>[3x]QDSTSDLIPAPPLSKVPLQQNFQDNQFQGKWYVVGLAGNAILREDKDPQKMYATIYEL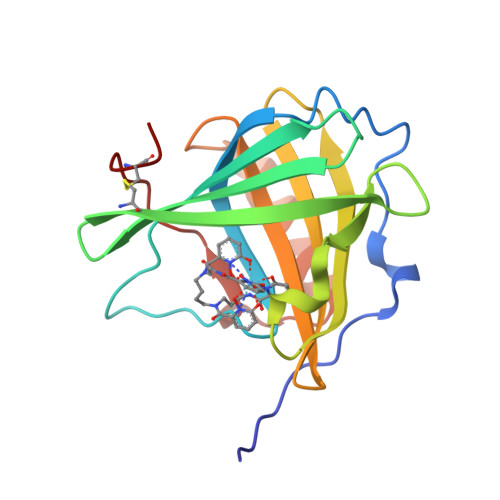KEDKSYNVTSVLFRKKKCDYWIRTFVPGSQPGEFTLGNIKSYPGLTSYLVRVVSTNYNQHAMVFFKKVSQNREYFKITLYGRTKELTSELKENFIRFSKSLGLPENHIVFPVPIDQCIDG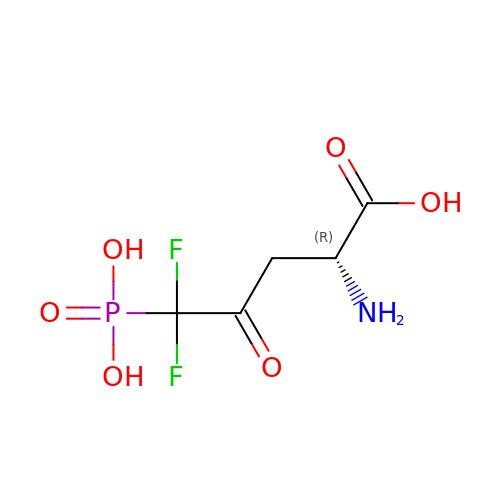5,5-difluoro-4-oxo-5-phosphono-D-norvaline | C5 H8 F2 N O6 P | WIAFNWXXJIHDPS-UWTATZPHSA-N(4R)-4-[4-(5-fluoro-1H-indol-3-yl)piperidine-1-carbonyl]piperidin-2-one 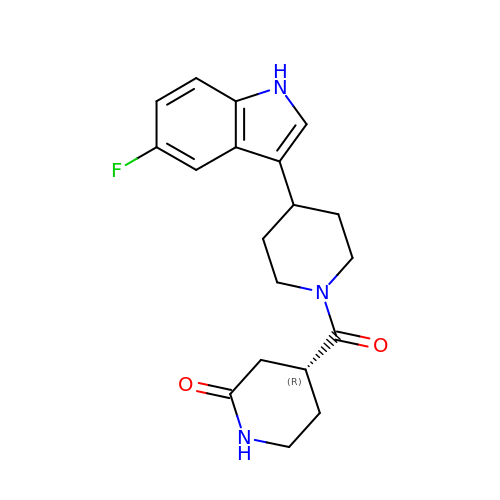| C19 H22 F N3 O2 | QDBIALQKWZMDJW-CYBMUJFWSA-N> MTDAVAGKTSLPPPVAIIVGHNIDASAMPLTYERNRFVIDMLQHYACPVFSHKKSGDAMNTVSSDVFEWVLEPFPVVGVEDMTAFHDRAYLNYLSIREALSEVDERASTVKPPLRVLPDLVPIPADEEYGLVNENMPFVGMWRTIQATVSGTLLAARLLAQPGRFAAIHWFGGRHHAKKSTAGGFCFANDVVLGVLELKKLLSSDKNGILVVDVDAHHGDGTQSAFLHDNSVLTLSMHAHGVGIFPGTGGIEEIGAGLGRGFTMNVPLPEGATDILAVTLMYRSIHFAFKKLGEGLAAIVIVCGSDALSGDPLGALNLTVGGMQSIIRLLLKEAARRSLKVLLLGAGGYVDTSCARLAGVVTKDVLSCAAAMRLGKTEYFGDSANLGDN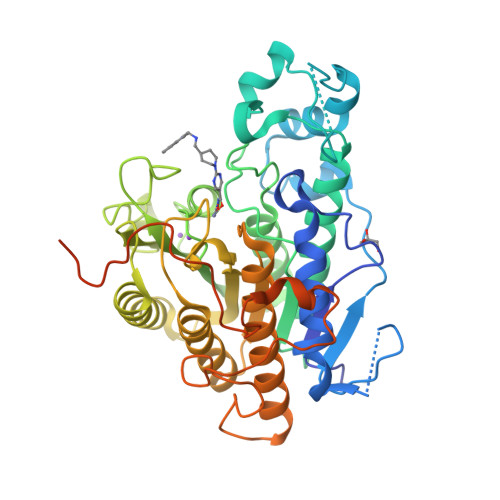LGVAVPEGCEYFTRYGPSFLMHGLPPARVSKLYRLPYGSPLFMRMQRAATKEALRRRLNQEQDEEEDAEDSGLEVLFQ> DDIKVAVVGAMSGPIAQWGDMEFNGARQAIKDINAKGGIKGDKLVGVEYDDACDPKQAVAVANKIVNDGIKYVIGHLCSSSTQPASDIYEDEGILMISPGATNPELTQRGYQHIMRTAGLDSSQGPTAAKYILETVKPQRIAIIHDKQQYGEGLARSVQDGLKAANANVVFFDGITAGEKDFSALIARLKKENIDFVYYGGYYPEMGQMLRQARSVGLKTQFMGPEGVGNASLSNIAGDAAEGMLVTMPKRYDQDPANQGIVDALKADKKDPSGPYVWITYAAVQSLATALERTGSDEPLAL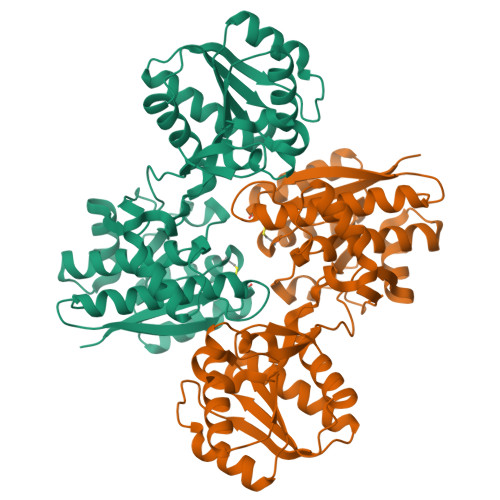VKDLKANGANTVIGPLNWDEKGDLKGFDFGVFQWHADGSSTKAK> AASCVLLHTGQKMPLIGLGTWKSEPGQVKAAVKYALSVGYRHIDCAAIYGNEPEIGEALKEDVGPGKAV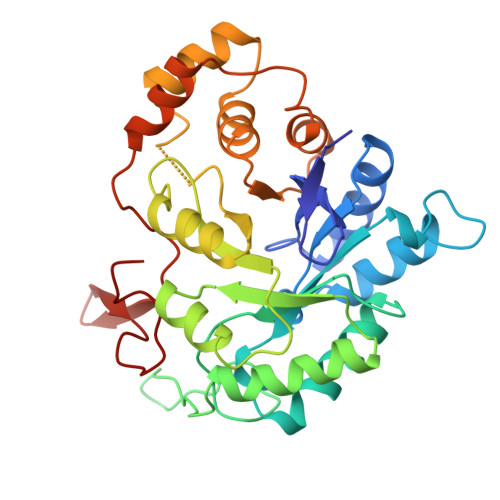PREELFVTSKLWNTKHHPEDVEPALRKTLADLQLEYLDLYLMHWPYAFERGDNPFPKNADGTICYDSTHYKETWKALEALVAKGLVQALGLSNFNSRQIDDILSVASVRPAVLQVECHPYLAQNELIAHCQARGLEVTAYSPLGSSDRAWRDPDEPVLLEEPVVLALAEKYGRSPAQILLRWQVQRKVICIPKSITPSRILQNIKVFDFTFSPEEMKQLNALNKNWRYIVPMLTVDGKRVPRDAGHPLYPFNDPY>MPINRPNLNLNIPPLNIVAAYDGAEIPSTNKHLKNNFNSLHNQMRKMPVSHFKEALDVPDYSGMRQSGFFAMSQGFQLNNHGYDVFIHARRESPQSQGKFAGDKFHISVLRDMVPQAFQALSGLLFSEDSPVDKWKVTDMEKVVQQARVSLGAQFTLYIKPDQENSQYSASF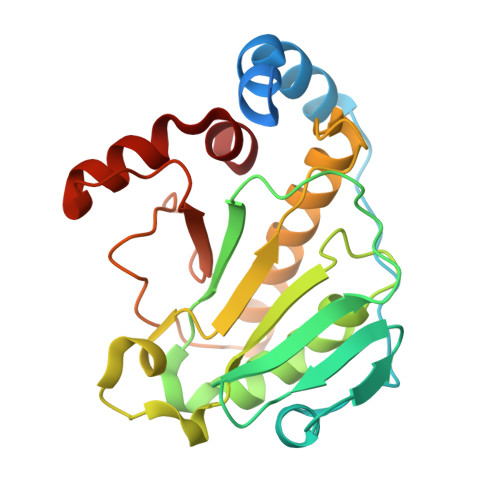LHKTRQFIECLESRLSENGVISGQCPESDVHPENWKYLSYRNELRSGRDGGEMQRQALREEPFYRLMTE[2x]>[2x]MDSKQQCVKLNDGHFMPVLGFGTYAPPEVPRSKALEVTKLAIEAGFRHIDSAHLYNNEEQVGLAIRSKIADGSVKREDIFYTSKLWSTFHRPELVRPALENSLKKAQLDYVDLYLIHSPMSLKPGEELSPTDENGKVIFDIVDLCTTWEAMEKCKDAGLAKSIGVSNFNRRQLEMILNKPGLKYKPVCNQVECHPYFNRSKLLDFCKSKDIV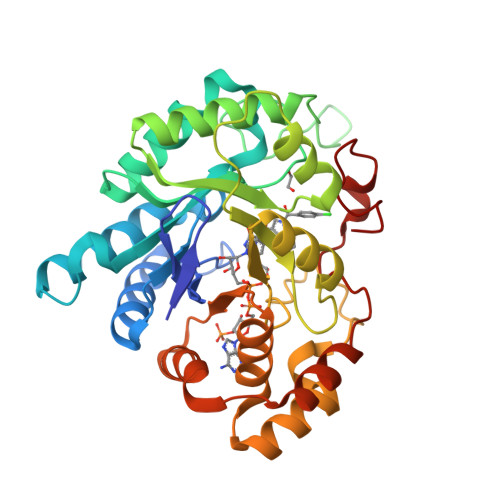LVAYSALGSQRDKRWVDPNSPVLLEDPVLCALAKKHKRTPALIALRYQLQRGVVVLAKSYNEQRIRQNVQVFEFQLTAEDMKAIDGLDRNLHYFNSDSFASHPNYPYSDEY5,5,5-TRIFLUORO-3-HYDROXY-4-[2-(5,5,5-TRIFLUORO-3-HYDROXY-4-{3-METHYL-2-[3-METHYL-2-(3-METHYL-BUTYRYLAMINO)-BUTYRYLAMINO]-BUTYRYLAMINO}-PENTANOYLAMINO)-PROPIONYLAMINO]-PENTANOIC 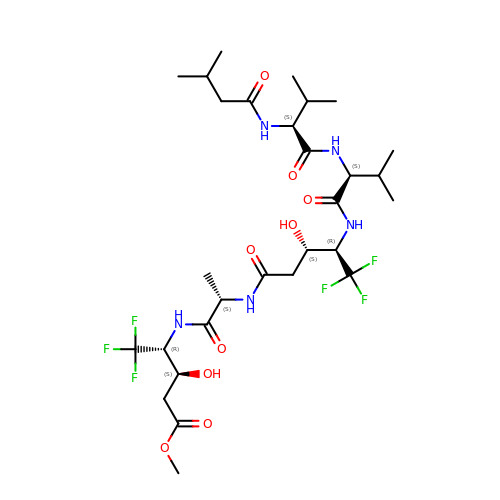ACID METHYL ESTER | C29 H47 F6 N5 O9 | DBMUWIXNLHQYDY-OCVHHRCCSA-N AppA, the Escherichia coli periplasmic phytase of clade 2 of the histidine phosphatase (HP2) family, has been well-characterized and successfully engineered for use as an animal feed supplement. The E. Coli periplasmic phytase, AppA, is a 1D-6-phytase (EC 3.1.3.2) and initial hydrolysis preferentially liberates the phosphate at the 1D-6-position on the inositol ring. HP2Ps catalyse the hydrolysis of phytate via an obligatory phosphohistidine intermediate. The catalytic proton donor is found in a second, short, conserved motif with sequence HD positioned such that the aspartic acid residue functions as the consensus proton donor in the catalytic mechanism.

The AppA-HET variant, which produces almost equal amounts of InsP5 [4/6-OH] and InsP5 [1/3-OH], shows the greatest reshaping of the active site. The structure reveals the glutamate residue to be found as the t rotamer (χ1 = 168°) pointing away from the substrate analogue, instead forming a salt bridge with H250 and making only weak interactions with the sulfates bound in pockets A and B. Furthermore, there is no low energy (or otherwise) rotamer described for glutamate which can leave its carboxyl group suitably positioned for to directly participate in catalysis. This is consistent with the low turnover number recorded for this variant. In fact, E304 positions its carboxylic group at the back of pocket B forming a salt bridge with His250 and makes only weak interactions with the sulfates bound in pockets A and B. A change in polarity also occurs in this pocket because of the distal position of the carboxylic acid group of E304. The sum of these changes presumably produces an active site able to accommodate multiple binding modes. However, the electron density for the InsS6 molecule bound to the active site of the AppA-HET variant was less well-defined. Given that this variant shows a reduced stereospecificity in hydrolysis of phytate it is possible that the enzyme may be able to bind the substrate analogue in multiple orientations. Consequently, the sulfomonoester groups at positions 1D-3 and 1D-6 of the inositol ring of InsS6 were simultaneously modelled in the primary specificity pocket adjacent to His17 to model static disorder in the binding of the inhibitor. The inhibitor molecules have refined occupancy ratios 0.47:0.53 (S3:S6) suggesting little intrinsic preference between the two orientations of binding. In addition, in the structure solved for the AppA-HET variant an inhibitor molecule was also found at the entrance of the active site, just above the inhibitor molecule occupying the catalytic site, and interacting with K24.

> GPQSEPELKLESVVIVSRHGVRAPTKATQLMQDVTPDAWPTWPVKLGWLTPRGGELIAYLGHYQRQRLVADGLLAKKGCPQSGQVAIIADVDERTRKTGEAFAAGLAPDCAITVHTQADTSSPDPLFNPLKTGVCQLDNANVTDAILSRAGGSIADFTGHRQTAFRELERVLNFPQSNLCLKREKQDESCSLTQALPSELKVSADNVSLTGAVSLASMLTEIFLLQQAQGMPEPGWGRITDSHQWNTLLSLHNAQFYLLQRTPEVARSRATPLLDLIKTALTPHPPQKQAYGVTLPTSVLFIAGHETNLANLGGALELNWTLPGQPDNTPPGGELVFERWRRLSDNSQWIQVSLVFQTLQQMRDKTPLSLNTPPGEVKLTLAGCEERNAQGMCSLAGFTQIVNEARIPACSL> TSMDPSSPNYDKWEMERTDITMKHKLGGGQYGEVYEGVWKKYSLTVAVKTLKEDTMEVEEFLKEAAVMKEIKHPNLVQLLGVCTREPPFYIITEFMTYGNLLDYLRECNRQEVNAVVLLYMATQISSAMEYLEKKNFIHRDLAARNCLVGENHLVKVADFGLSRLMTGDTYTAHAGAKFPIKWTAPESLAYNKFSIKSDVWAFGVLL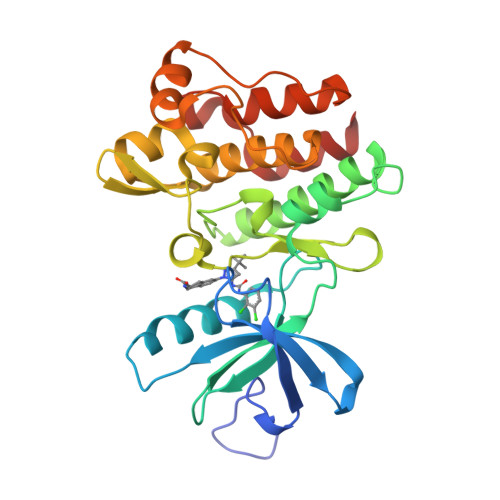WEIATYGMSPYPGIDLSQVYELLEKDYRMERPEGCPEKVYELMRACWQWNPSDRPSFAEIHQAFETMFQE> MSSKYPRSVRRCLPLWALTLEAALILLFYFFTHYDASLEDQKGLVASYQVGQDLTVMAALGLGFLTSNFRRHSWSSVAFNLFMLALGVQWAILLDGFLSQFPPGKVVITLFSIRLATMSAMSVLISAGAVLGKVNLAQLVVMVLVEVTALGTLRMVISNIFNTDYHMNLRHFYVFAAYFGLTVAWCLPKPLPKGTEDNDQRATIPSLSAMLGALFLWMFWPSVNSPLLRSPIQRKNAMFNTYYALAVSVVTA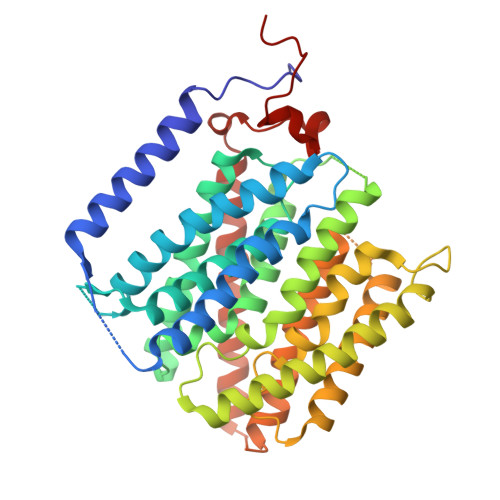ISGSSLAHPQRKISMTYVHSAVLAGGVAVGTSCHLIPSPWLAMVLGLVAGLISIGGAKCLPVCCNRVLGIHHISVMHSIFSLLGLLGEITYIVLLVLHTVWNGNGMIGFQVLLSIGELSLAIVIALTSGLLTGLLLNLKIWKAPHVAKYFDDQVFWKFPHLAVGF5'-[(3-{[(4-tert-butylphenyl)carbamoyl]amino}propyl)(propan-2-yl)amino]-5'-deoxyadenosine 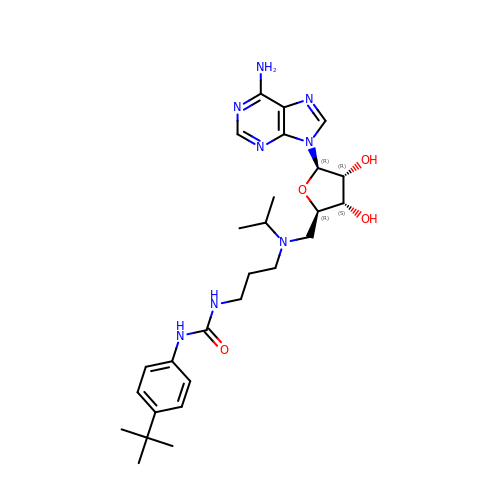| C27 H40 N8 O4 | MTLMDZJUGDUTCP-PTGPVQHPSA-N> MASPVIYQAEDAIIYNAILETVNAGYTGSCYVNYHNEVGGYIEWNVNAPSSGSYALIFRYANGTTANRPMRITVNGNIVKPSMDFVSTGAWTTWNEAGIVANLNQGNNVIRATAIASDG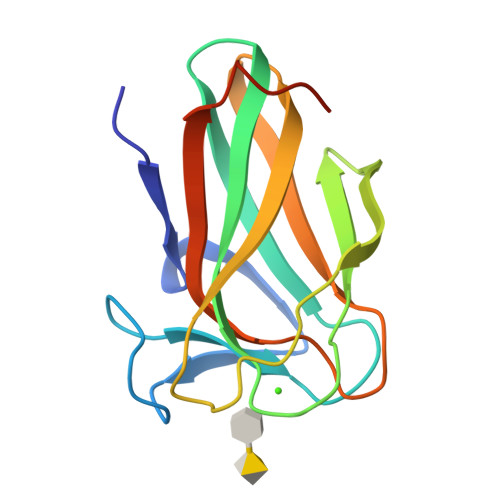GPNVDYLKVFSANAFQPLEHHHHHH2,6-dichloro-N-[(2R)-2-(5,6-dimethyl-1H-benzimidazol-2-yl)-2-phenylethyl]-4-(4H-1,2,4-triazol-4-yl)benzamide 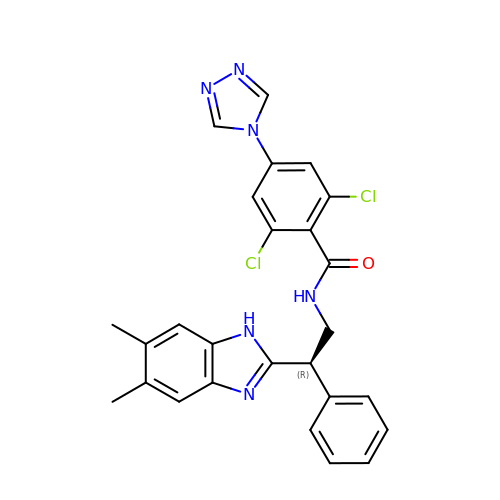| C26 H22 Cl2 N6 O | KSIMBQNDIBGKTO-IBGZPJMESA-N> EVNKIIGSRTAGEGAMEYLIEWKDGHSPSWVPSSYIAADVVSEYETPWWTAARKADEQALSQLLEDRDVDAVDENGRT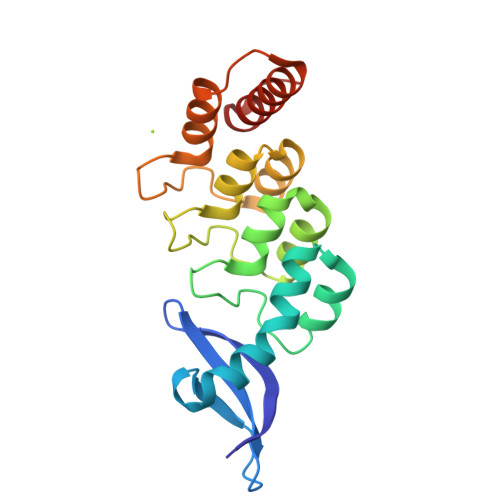ALLFVAGLGSDKCVRLLAEAGADLDHRDMRGGLTALHMAAGYVRPEVVEALVELGADIEVEDERGLTALELAREILKTTPKGNPMQFGRRIGLEKVINVLEGQVF> MKINRQQYAESYGPTVGDQVRLADTDLWIEVEKDYTTYGDEANFGGGKVLREGMGENGTYTRTENVLDLLLTNALILDYTGIYKADIGVKDGYIVGIGKGGNPDIMDGVTPNMIVGTATEVIAAEGKIVTAGGIDTHVHFINPDQVDVALANGITTLFGGGTGPAEGSKATTVTPGPWNIEKMLKSTEGLPINVGILGK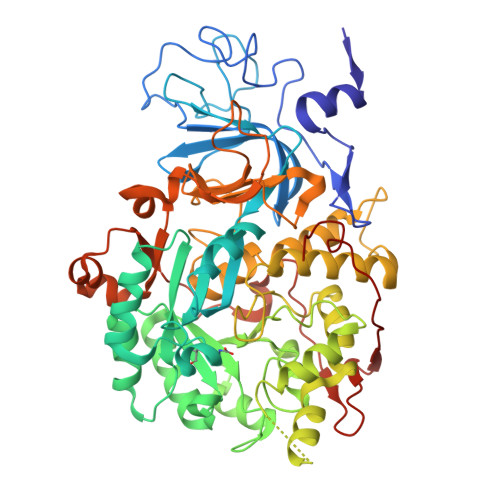GHGSSIAPIMEQIDAGAAGLKIHEDWGATPASIDRSLTVADEADVQVAIHSDTLNEAGFLEDTLRAINGRVIHSFHVEGAGGGHAPDIMAMAGHPNVLPSSTNPTRPFTVNTIDEHLDMLMVCHHLKQNIPEDVAFADSRIRPETIAAEDILHDLGIISMMSTDALAMGRAGEMVLRTWQTADKMKKQRGPLAEEKNGSDNFRAKRYVSKYTINPAIAQGIAHEVGSIEEGKFADLVLWEPKFFGVKADRVIKGGIIAYAQIGDPSASIPTPQPVMGRRMYGTVGDLIHDTNITFMSKSSIQQGVPAKLGLKRRIGTVKNCRNIGKKDMKWNDVTTDIDINPETYEVKVDGEVLTCEPVKELPMAQRYFLF methyl alpha-D-glucopyranoside 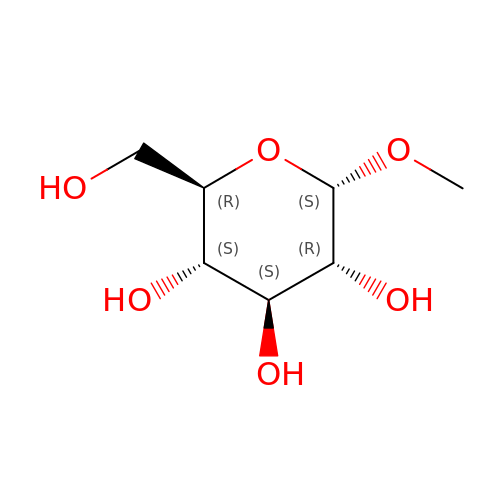| C7 H14 O6 | HOVAGTYPODGVJG-ZFYZTMLRSA-N[(R)-(4-fluorophenyl)-[[(2S)-2-methyl-3-sulfanyl-propanoyl]amino]methyl]boronic acid 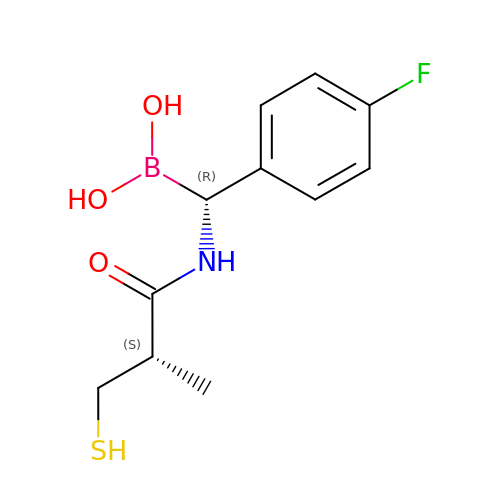| C11 H15 B F N O3 S | CDDJMEDWZMPIRW-XCBNKYQSSA-N>PSVYDAAAQLTADVKKDLRDSW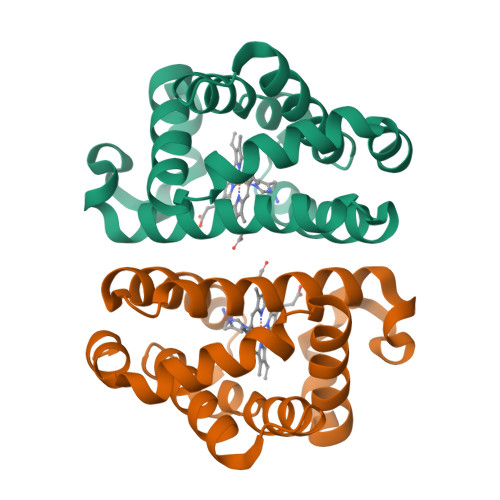KVIGSDKKGNGVALMTTLFADNQETIGYFKRLGDVSQGMANDKLRGHSITLMYALQNYIDQLDNPDDLVCVVEKFAVNHITRKISAAEFGKINGPIKKVLASKNFGDKYANAWAKLVAVVQAAL[2x]> QPIFLNVLEAIEPGVVCAGHDNNQPDSFAALLSSLNELGERQLVH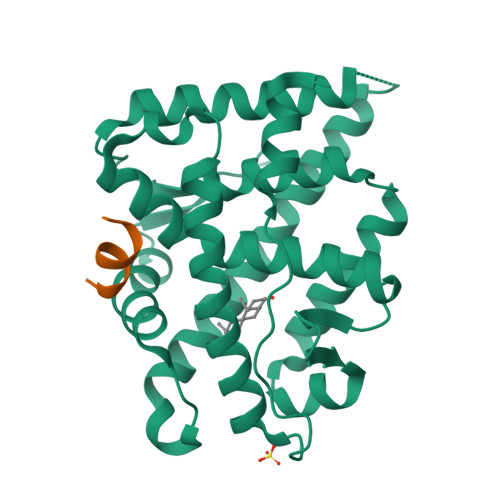VVKWAKALPGFRNLHVDDQMAVIQYSWMGLMVFAMGWRSFTNVNSAMLYFAPDLVFNEYRMHKSRMYSQCVRMRHLSQEFGWLQITPQEFLCMKALLLFSIIPVDGLKNQKFFDELRMNYIKELDRIIACKRKNPTSCSRRFYQLTKLLDSVQPIARELHQFTFDLLIKSHMVSVDFPEMMAEIISVQVPKILSGKVKPIYFHTQ;> SDSAFSRLYTRS To gain insight into the evolution and designability of ligand binding and specificity, we analyzed the homologous PBPs, PotF and PotD, which are Escherichia coli putrescine (PUT)-binding protein and spermidine (SPD)-binding protein, respectively. They constitute the first elements of two separate multicomponent uptake systems (PotFGHI and PotABCD) to transport the cationic polyamines PUT and SPD across the cellular membrane. Still, the protein-binding modes differ: PotF shows affinity for PUT and SPD, whereas PotD exclusively binds SPD. Prior to this work, we grafted the seven differences in amino acids from PotD binding pocket onto PotF; this resulted in PotF_SPD, which will be referred to as PotF/D throughout this work to keep naming for mutants more concise.

We introduced the S247D exchange into PotF/D and into our high-affinity constructs E39D–Y87S–F88Y and E39D–F88A/L. The combination of S247D with the other constructs led to an affinity improvement with which the nanomolar range was reached for the first time, while keeping the order of affinities in the different mutants the same compared with the prior analysis. We successfully obtained X-ray data for all newly generated variants including the F88A carrying construct. All structures but PotF/D–S247D adopt a fully closed wildtype conformation. In the F88L/A variants, Y87 is finally able to rotate toward the binding pocket and allows distal salt bridge formation. The orientation of the residues in both mutants is identical, confirming the F88L containing variant as a structural example for the noncrystallizable F88A construct in the first part of this study. An interesting feature of the F88A containing construct is the orientation of the N2 of SPD, as it faces toward the aromatic box residues to form stacking interaction in contrast to all other constructs, in which interaction with D278 is always preferred. The F88A containing structure is less resolved than the others, and the ligand density could allow for both conformations of N2 in the density, but multiple refinement cycles ended up preferring the built one. In all constructs that carry S247D, SPD adopts a “relaxed” conformation and does not show unexpected bending of its backbone to fit a specific position as it does when being bound by PotF wildtype or PotF/D.

>[2x]AEQKTLHIYNWTDYIAPDTVANFEKETGIKVVYDVFDSNEVLEGKLMAGSTGFDLVVPSAYALERQLTAGVFQPLDKSKLPEWKNLDPELLKLVAKHDPDNKFAMPYMWATTGIGYNVDKVKAVLGENAPVDSWDLILKPENLEKLKSCGVSFLDDPEEVFATVLNYLGKDPNSTKADDYTGPATDLLLKLRPNIRYFHSSQYINDLANGDICVAIGWAGDVWQASNRAKEAKNGVNVSFSIPKEGAMAWFDVFAMPADAKNKDEAYQFLNYLLRPDVVAHISDHVFYANANKAATPLVSAEVRENPGIYPPADVRAKLFTQKVQDPKIDRVRTRAWTKVKSGKLEHHHHHH> MDRINESHQRFLQALMSHGIMEGSAVRALHRHCCELHKVHYMHDKLDDFVGVLNRHLQPLFMTIEKGVGEEDGLTYYALVNRVENDITKMASDYAENELELFRKTMELIILSDNGFATSISILNLADELQSKKMKKKEVEQLLQSFVQEKWLIGRNGEYTLHTRCIMELEHYIRNTYQDVAKICNVCRKVAIQSQLCENCGIPLHLQCAGKYFHGKANPTCPNCNESWPHEIPDLNQVSSQGPSHSQ;> MQNHSQEQVNLKVGEVVQYLLIKD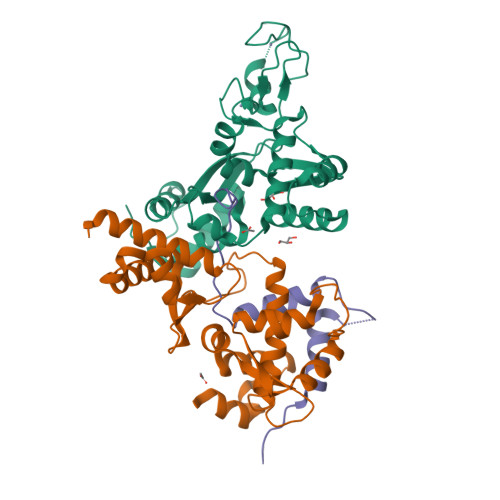QKKLPIKRADIVRSVIKEYKDIYPEIIHRAQITLQQVFGFQLEEIDTKSHIYILTNKLQRVQGDGMRVDENTSKLGLLMVILSLIFMKGNTAKESAIWEMLRRLRIEPGEMHSEFGDVKKLVTEEFVKQKYLEYNKVPHIDPVEYEFRWGQRAFKETSKMKVLEFVSKIQQKDPKSWTTQYKDAQEQTQVAGR;> GSHMTVFDPTSFTADLLSFMGLNRMESPGHNSANESDDEGYAGGYLPTDAWQKLGSEAENYFKRTPTFHFMLGSFKTEP> MNTFSSPPNVIREYNDSTYQSPLNSQFHQSPFLQTQSPDYVSLREEEDDNNDKNLDIMSSCIVDSVIYKSQKIAGPLLSQISNLNIQQALIIRELLFTLLGHEGHYIQYSKRYDPTSQISRIEGPDYKIAKNLDISLKVITKKLVKFGKFYSGLKSFIQVFDNNKFGKIVQKFCSEVRKFLSSYQQVLINVEHEF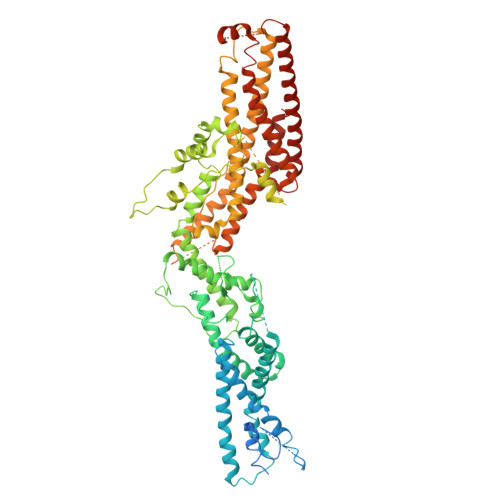KFNKNFNLNMLDSLLHQEISNEMTHLYQIGIEISRITEERQKMSQAEIMGNFEPTTLANTSMNGINSEPNLYYGKFDCCKGGLLLQVIQERMVYYKGDPTSLDFLTQLFDIVSSDYIGMLNQWLLEGVINDPFDEFMIREKRVPDSFMEIFQSKSEYYWNELFLIKIDGLLNQFQNSTIQSKILNTGKYLNIFKRCTGLHNFESLKEKLTTITSLAAPDLELKIDEFYHRANKMLMKLLFDGYNFPSVVNIFQRLFLFADSFQIDNFIDSTFSELKRGKLKISVSRLQKQYDDIFKEKIENKVGVRPSVYDVLKKNQKLSVTSESLYKVVEELMEKNSDYLISDNNLRGIFHRVASLRDDSRLTISSTADSATENVKDEPTITSVDLTIPLPFPLNLVLNQQLSYQYEIMFKLLINIKFISKYNSSNWQEMNYSKIWTNSHFNSSVKKWILRCRVLHSRICSFIHELENYIVHDVIEHNFEEIKNLIHTTATNLATSELGSDINDEGDNIFNGSLIRGTFNNNSIFDSKVHKHRTTTYVEGISTVEQLIQKFLDYSSTLLNDSLLTREESLRQLRKMLDFIFHFNNYIVQVKKVLVLLNHELFNEYSKEFPTKFEKPMDQESIDKRFANLSDTFLMQYEKFGENLVTFLATIKQVGERENQGLLELSNRLELCFPE>GAMPHDPSFTPTQLAARAAYLLRGNDLGTMTTAAPLLYPHMWSWDAAFVAIGLAPLSVERAVVELDTLLSAQWRNGMIPHIVFANGVDGYFPGPARWATATLADNAPRNRLTSGITQPPVHAIAVQRILEHARTRGRSTRAVAEAFLDRRWGDLMRWHRWLAECRDRNERGRITLYHGWESGMDNSPRWDSAYANVVPGKLPEYQRADNVIITDPSQRPSDGEYDRYLWLLEEMKAVRYDDERLPSVMSFQVEDVFFSAIFSVACQVLAEIGEDYKRPHADVKDLYLWAERFRAGVVETTDQRTGAARDFDVLAEKWLVTETAAQFAPLLCGGLPHDRERALLKLLEGPRFCGHPDLKYGLIPSTSPVSRDFRPREYWRGPVWPVLTWLFSWCFARRGWAERARLLRQEGLRQASDGSFAEYYEPFTGEPLGSMQQSWTAAAVLDWLG[4x]

A glucosylglycerate hydrolase (GgH) identified in M. hassiacum and found to be highly conserved among rapidly growing mycobacteria is likely to be responsible for the rapid mobilization of GG accumulated during nitrogen starvation by hydrolysing it to glucose and glycerate. The MhGgH monomer displays an (α/α)6-barrel domain typical of glycoside hydrolase family 63 (GH63), to which MhGgH belongs. While the active site of GH63 members acting on larger substrates is located in an open, solvent-accessible cleft, those of MhGgH and of MgH from T. thermophilus are covered by a cap domain (subdivided into A′- and B′-regions) with constrained access through a narrow negatively charged tunnel. The crystallographic structure of MhGgH revealed a homotetrameric architecture, which is compatible with the oligomeric organization of the enzyme in solution as assessed by SAXS.

Despite crystallizing in the same conditions, selenomethionine-substituted MhGgH produced monoclinic crystals (space group P21) that were used for structure solution by multi-wavelength anomalous diffraction at the K absorption edge of selenium. The total surface area of each monomer is ∼17 300 Å2, of which ∼1600 Å2 is buried in intermonomer contacts. The largest interface area (∼900 Å2) occurs between molecules A and C (interface A:C) and molecules B and D, and involves 14 (A:C) or 12 (B:D) hydrogen bonds. With approximately half of the size (∼480 Å), the interface between dimers A:B and C:D is stabilized by four salt bridges. The smallest interface occurs between molecules A and D (and molecules B and C), with a buried surface of ∼260 Å2 and a single hydrogen bond. The C-terminus of each MhGgH monomer is in the close vicinity of the A:C (or B:D) interface and the addition of the C-terminal affinity tag is likely to disrupt dimer–dimer association and impact the quaternary organization of the enzyme, which is in line with the observed lower maximum temperature of activity and decreased stability of the MhGgH-His6 variant.>[4x]MKPERKRVSKLMAYILRHSPEEFGLRPDVEGFVSLNELVNALKTVYPEVTEEFVREIVENDPKGRYEIRGDRIRARYGHSFPVSLDHEEDTESRFLYHGT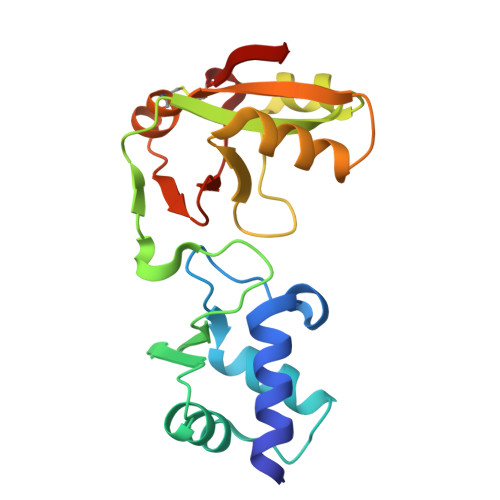PRRNLPSILKEGLKPMKRQYVHVSTDKIEALETGRRHGREVVLLVIDAECLRKRGFKIYKAGKNVRIVERVPPDCITLAV> GSSHHHHHHSSGLVPRGSMSTSWSDRLQNAADMPANMDKHALKKYRREAYHRVFVNQSLAMEKIKCFGFNMDYTLAVYKSPEYESLGFELTVERLVSIGYPQELLSFAYDSTFPTRGLVFDTLYGNLLKVDAYGNLLVCAHGFNFIRGPETREQYPNKFIQRDDTERFYILNTLFNLPETYLLACLVDFFTNCPRYTSCETGFKDGDLFMSYRSMFQDVRDAVDWVHYKGSLKEKTVENLEKYVVKDGKLPLLLSRMKEVGKVFLATNSDYKYTDKIMTYLFDFPHGPKPGSSHRPWQSYFDLILVDARKPLFFGEGTVLRQVDTKTGKLKIGTYTGPLQHGIVYSGGSSDTICDLLGAKGKDILYIGDHIFGDILKSKKR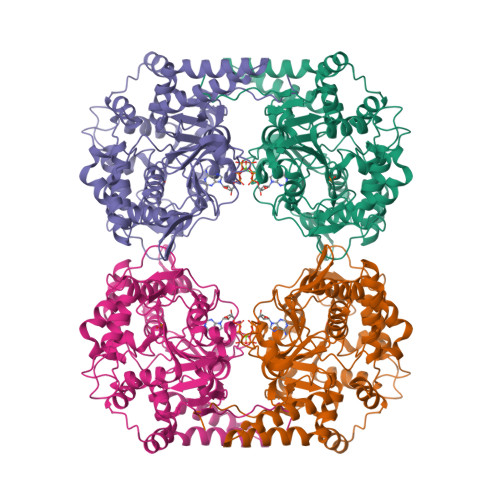QGWRTFLVIPELAQELHVWTDKSSLFEELQSLDIFLAELYKHLDSSSNERPDISSIQRRIKKVTHDMDMCYGMMGSLFRSGSRQTLFASQVMRYADLYAASFINLLYYPFSYLFRAAHVLMPHESTVEHTHVDINEMESPLATRNRTSVDFKDTDYKRHQLTRSISEIKPPNLFPLAPQEITHCHDEDDDEEEEEEEE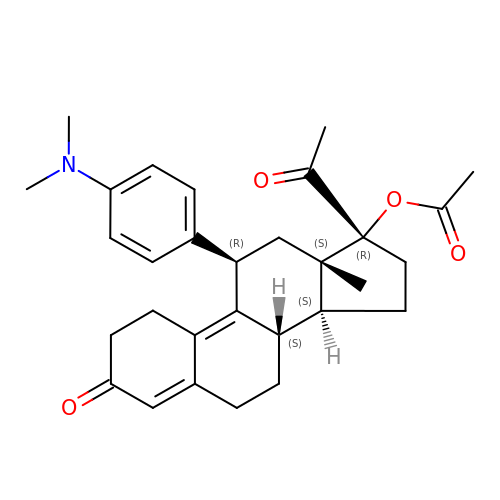[(8S,11R,13S,14S,17R)-17-acetyl-11-[4-(dimethylamino)phenyl]-13-methyl-3-oxo-1,2,6,7,8,11,12,14,15,16-decahydrocyclopenta[a]phenanthren-17-yl] acetate | C30 H37 N O4 | OOLLAFOLCSJHRE-ZHAKMVSLSA-N> MENTENSVDSKSIKNLEPKIIHGSESMDSGISLDNSYKMDYPEMGLCIIINNKNFHKSTGMTSRSGTDVDAANLRETFRNLKYEVRNKNDL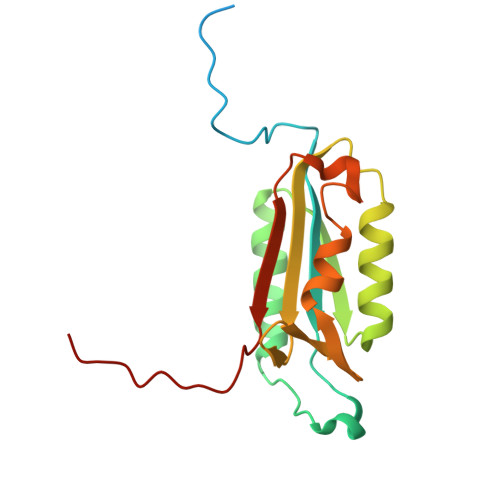TREEIVELMRDVSKEDHSKRSSFVCVLLSHGEEGIIFGTNGPVDLKKITNFFRGDRCRYLTGKPKLFIIQACRGTELDCGIETD>[2x]MSDAAPSLSNLFYDPTYNPGQSTINYTSIYGNGSTITFDELQGLVNSTVTQAIMFGVRCGAAALTLIVMWMTSRSRKTPIFIINQVSLFLIILHSALYFKYLLSNYSSVTYALTGFPQFISR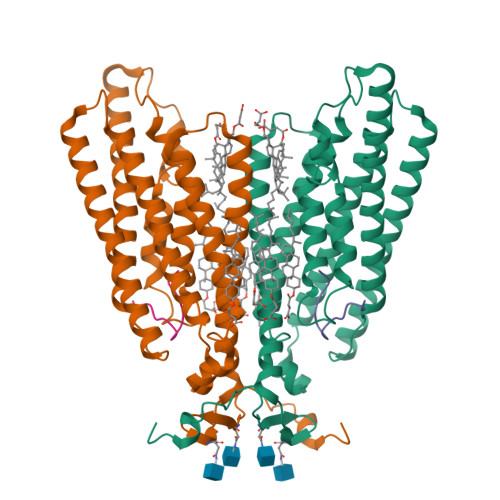GDVHVYGATNIIQVLLVASIETSLVFQIKVIFTGDNFKRIGLMLTSISFTLGIATVTMYFVSAVKGMIVTYNDVSATQDKYFNASTILLASSINFMSFVLVVKLILAIRSRRFLGLKQFDSFHILLIMSCQSLLVPSIIFILAYSLKPNQGTDVLTTVATLLAVLSLPLSSMWATAANNASKTNTITSDFTTSTDRFYPGTLSSFQTDSINNDAKSSLRSRLYDLYPRRKETTSDKHSERTFVSETADDIEKNQFYQLPTPTSSKNTRIGPFADASYKEGEVEPVDMYTPDTAADEEARKFWTEDNNNL;>[2x]WHWLQLKPGQPMY The transcription factors p53, p63 and p73 play an important role in cancer prevention, development and longevity. The three proteins share a similar domain organization, being composed of structured DNA-binding domain (DBD) and tetramerization domain flanked by intrinsically disordered regions. Tetramers are formed via a short tetramerization domain that follows the DBD, with a short flexible linker region separating the two domains. Here, we report crystal structures of different p63 tetramerization domain variants, showing not only marked similarity to p73 but also small differences that may be important for regulating the function of p63 in vivo.

In addition, we also solved the structure of a variant lacking the C-terminal helix altogether, that is, containing only the structural elements of the canonical p53 tetramerization domain motif. Deletion of the H2 helix has been shown to substantially destabilize the p63 and p73 tetramers, and much higher protein concentrations were needed to shift the equilibrium toward tetrameric species. We solved the crystal structure of such a truncated variant of p63, p63(359–388), at a resolution of 1.9 Å. Interestingly, this crystal structure, solved in the space group P1, contained one tetramer in the asymmetric unit but with fundamentally different packing characteristics than those observed for the longer variant. The primary dimers are formed as observed for the longer variant, that is, by formation of an intermolecular β-sheet and antiparallel packing of the H1 helices. These primary dimers, however, pack in an antiparallel fashion to form tetramers, which is in stark contrast to the orthogonal packing observed in the full-length tetramers of p53, p63 and p73. In addition, there are small differences in the structure of the primary dimers, most notably, a difference in packing angle and conformation of the H1 helix. This helix adopts an α-helical conformation throughout, whereas the packing interactions in the full-length variant cause a distortion at the C-terminal end of the helix and a transition to a 310-helical conformation. Key hydrophobic interactions at the center of the primary dimer interface are conserved. Hence, loss of the second helix in p63 and p73 not only weakens the tetramer but also fundamentally alters the overall orientation of the H1 helix packing, revealing a high degree of fluidity of this interface in the absence of the H2 helix.

>GSDELLYLPVRGRETYEMLLKIKESLELMQYL[4x]>[3x]ALPQTVRIGTDTTYAPFSSKDAKGEFIGFDIDLGNEMCKRMQVKCTWVASDFDALIPSLKAKKIDAIISSLS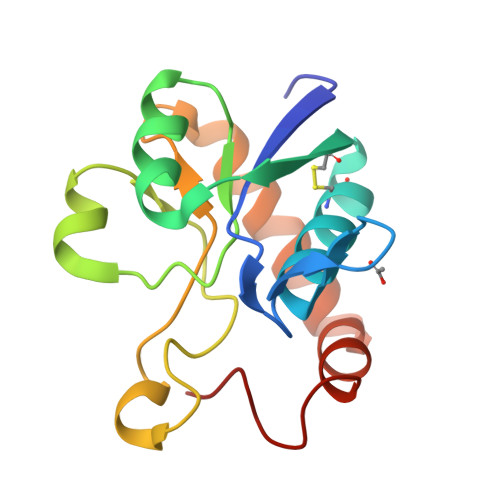ITDKRQQEIAFSDKLYAADVKDKKYFGDGTGVGLRKDDTELKAAFDKALTELRQDGTYDKMAKKYFDFNVYGD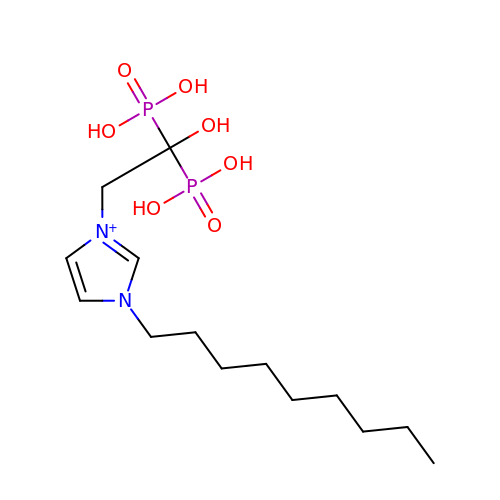[1-hydroxy-2-(1-nonyl-1H-3lambda~5~-imidazol-3-yl)ethane-1,1-diyl]bis(phosphonic acid) | C14 H29 N2 O7 P2 | ANVJZSKZYXLDSP-UHFFFAOYSA-O4-epi-vancosamine | C7 H15 N 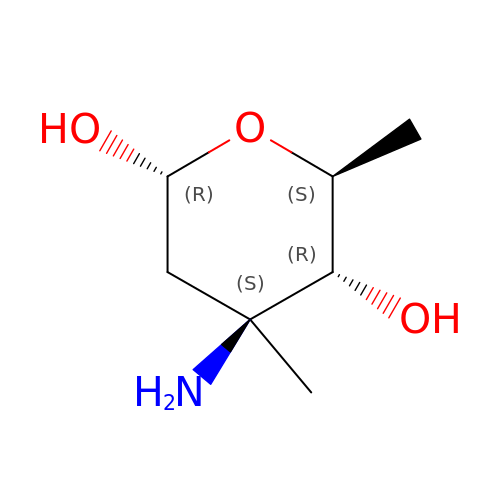O3 | OIJZDPGKNVKVBL-VZFHVOOUSA-N> MITHRPRGIEHPYARSLDQLYPAIPIAGQSLTIGATTSGPCSRMRCFVLWPEHEQVFDMSPVNGTDSDAALLAGGEGHLAAAQQAALDADNGWQTSIPHLPDQDATYYFEALTLDGRTETSESFPLTPSHWSAEPVGHIDIDGDRFIPDSPLWLVSSAGTHRVKFALRIEGDEHVVGFGERYDQLDQRGLRLDSVVFEQYKAQGKHHRTYLPMPFAQVVNEAGRAWGFHVETTRRTWYDVAATVSDRILIEVDLGFEAEKTPVVRVNTWSGSPTDVLNGFLDVAGRPAEMPEWIFGLWASGNEWNTQSLVMEQMDRHRNEGIPVSVVVIEAWSDEEGFTIFRDARYVPNQ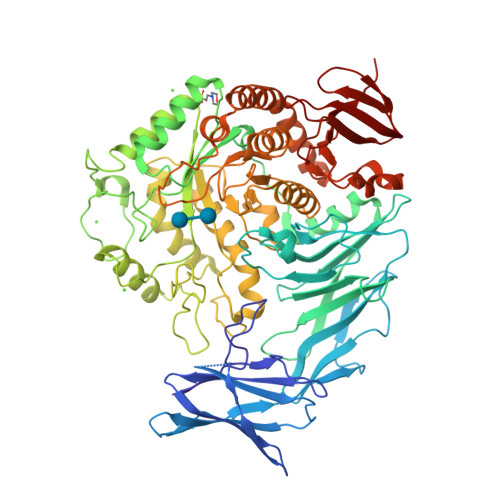GQPHRGPDFTYPSDGAWPDPAGMIRELHERGIRVILWQIPLQKTDDDLGPEALAQGNALIASGHVVKEPDGTPYKNRGWWFPNALMPDLSTEAGRQWWTEQRRYLVEDLDIDGFKTDGGEHAWGSDLRYEDGRRGDEGNNLYPVNYARAYGDLLRSAGKYPVTFSRSGFTGSQAHGLYWAGDEDSTWEAFRSSITAGITAGACGILYWGWDLAGFSGPVPEAELYARAFAAATFMPIMQYHSEFHHHELPLRDRTPWNVAEQTGCGELIDLARHYTRVREALRPYLVAQTRQCLQTGKPLMRAMFYDHADDPEIWAHPRQYMLGDELLINPVTAPGATTWTTYLPEGQWEDYWSGEVSEGGHLVTRAVGWDIIPVYRRVGAAL Sec4p is among the 11 Rab GTPases identified in S. cerevisiae and acts on the surface of membranes to regulate transport between the Golgi apparatus and the plasma membrane. To complete the cycle, the protein is reactivated by switching the guanine nucleotide state from GDP to GTP in a process stimulated by guanine nucleotide exchange factors (GEFs). Therefore, the structural and functional analysis of the mutant Ser29Val of Sec4p offers an opportunity to understand not just the basic differences between Ras GTPase families but also how Sec4p is activated during its GTPase cycle by its GEF Sec2p. Sec2p is a highly efficient exchange factor of Sec4p that stimulates nucleotide exchange by binding to the switch regions of Sec4p and altering its conformation resulting in decreased affinity between Sec4p and nucleotide. In this work we have investigated the nucleotide exchange mechanism of the Rab GTPase Sec4p and how its GEF Sec2p stimulates nucleotide dissociation, making use of the Sec4p mutant S29V corresponding to Gly12 in Ras proteins.

In contrast, the addition of GDP and magnesium does not disrupt the complex between Sec4pV29 and Sec2p. This enabled us to obtain crystals for the ternary complex Sec4pV29.GDP.Sec2p and solve the structure at 2.9 Å resolution. As seen in the other two structures of the complex Sec4p.Sec2p the average temperature factor is very high (66.8 Å2) which reflects the high flexibility of the complex. However, the presence of the nucleotide is confirmed by the OMIT map at 3σ. Superposition with previously solved structures of the complex Sec4p.Sec2p reveals that Sec4pV29.GDP.Sec2p shares high similarity with the Sec4p.Sec2p complex bound to phosphate with a RMSD between the 353 Cα atoms of 0.675 Å. However, due to the presence of the guanine ring the loop β6-α5 adopts a conformation that resembles the Sec4p.GDP and Sec4p.GTP structures. When the superposition between Sec4pV29.GDP.Sec2p and Sec4p.Phosphate.Sec2p structures is performed using only the Cα atoms of the Sec4p binding site of Sec2p (residues 100–120), it is clear that the mutant active site is in a more closed conformation than the wild type. Both the P-loop and the nucleotide are shifted in about 1 Å towards the SWI region in the V29 structure. We analyzed the crystal structure for the complex Sec4pV29 and Sec2p and determined that the complex was bound to a GDP molecule. This complex most likely represents the intermediate state of the nucleotide dissociation just before nucleotide release. We can predict that this difference would make magnesium rebinding to the intermediate state of the complex more difficult and together with the increase in the affinity for the nucleotide it could explain why the GDP bound state of Sec4pV29 can form a stable complex with Sec2p.

> SSIMKILLIGDVGVGKSCLLVRFVEDKFNPSFITTIGIDFKIKTVDINGKKVKLQLWDTAGQERFRTITTAYYRGAMGIILVYDVTDERTFTNIKQWFKTVNEHANDEAQLLLVGNKSDMETRVVTADQGEALAKELGIPFIESSAKNDDNVNEIFFTLAKLIQEKIDSN;>[2x]SNYNQLKEDYNTLKRELSDRDDEVKRLREDIAKENELRTKAEEEADKLNKEVEDLTASLFDEANNMVADARKEKYAIEILNKRLTEQLREKDT> SELFIVRQLLQIVKQKTNQNSVDTTLKFTLSALWNLTDESPTTCRHFIENQGLELFMRVLESFPTESSIQQKVLGLLNNIAEVQELHSELMWKDFIDHISSLLHSVEVEVSYFAAGIIAHLISRGEQAWTLSRSQRNSLLDDLHSAILKWPTPECEMVAYRSFNPFFPLLGCFTTPGVQLWAVWAMQHVCSKNPSRYCSMLIEEGGLQHLYNIKDHEHT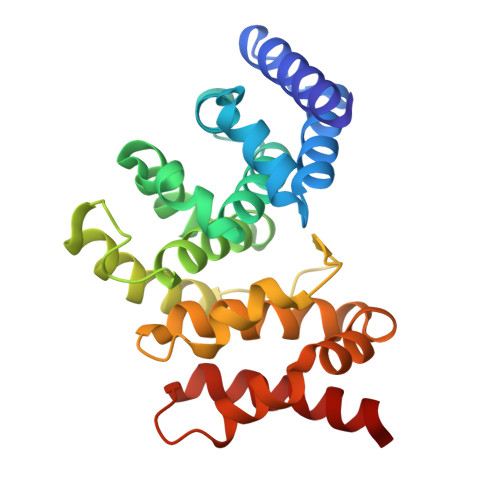DPHVQQIAVAILDSLEKHIVR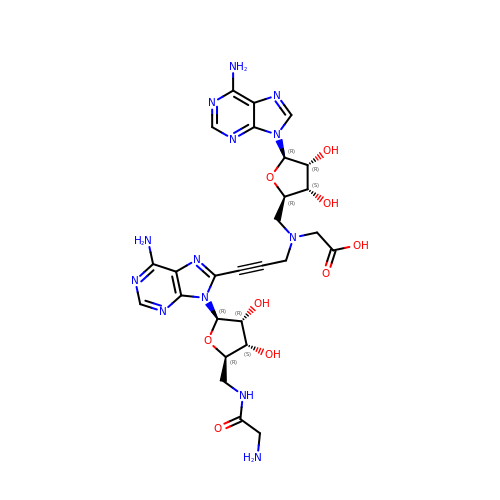2-[[(2~{R},3~{S},4~{R},5~{R})-5-(6-aminopurin-9-yl)-3,4-bis(oxidanyl)oxolan-2-yl]methyl-[3-[6-azanyl-9-[(2~{R},3~{R},4~{S},5~{R})-5-[(2-azanylethanoylamino)methyl]-3,4-bis(oxidanyl)oxolan-2-yl]purin-8-yl]prop-2-ynyl]amino]ethanoic acid | C27 H33 N13 O9 | NHPRQGWVLUQCPR-WNZAMUCISA-N>[3x]MNYNNKILVSESGLSQKHLIHGDEELFQHELKTIFARNWLFLTHDSLIPAPGDYVTAKMGIDEVIVSRQNDGSIRAFLNVCRHRGKTLVSVEAGNAKGFVCSYHGWGFGSNGELQSVPFEKDLYGESLNKKCLGLKEVARVESFHGFIYGCFDQEAPPLMDYLGDAAWYLEPMFKHSGGLELVGPPGKVVIKANWKAPAENFVGDAYHVGWTHASSLRSGESIFSSLAGNAALPPEGAGLQMTSKYGSGMGVLWDGYSGVHSADLVPELMAFGGAKQERLNKEIGDVRARIYRSHLNCTVFPNNSMLTCSGVFKVWNPIDANTTEVWTYAIVEKDMPEDLKRRLADSVQRTFGPAGFWESDDNDNMETASQNGKKYQSRDSDLLSNLGFGEDVYGDAVYPGVVGKSAIGETSYRGFYRAYQAHVSSSNWAEFEHASSTWHTELTKTTDR;>MMINIQEDKLVSAHDAEE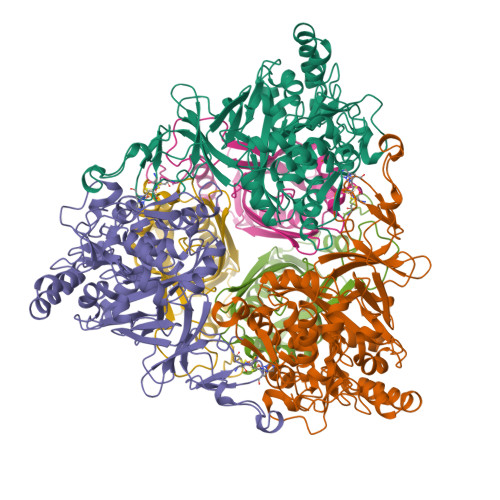ILRFFNCHDSALQQEATTLLTQEAHLLDIQAYRAWLEHCVGSEVQYQVISRELRAASERRYKLNEAMNVYNENFQQLKVRVEHQLDPQNWGNSPKLRFTRFITNVQAAMDVNDKELLHIRSNVILHRARRGNQVDVFYAAREDKWKRGEGGVRKLVQRFVDYPERILQTHNLMVFL[3x]> KVTLYKTTATADSDKFKISQILTFNFIKDKSYDKDTLVLKATGNINSGFVKPNPNDYDFSKLYWGAKYNVSISSQSNDSVNVVDYAPKNQNEEFQVQNTLGYTFGGNTAFSETINYKQESYRTTLSRNTNYKNVGWGVEAHKIMNNGWGPYGRDSFHPTYGNELFLAGRQSSAYAGQNFIAQHQMPLLSRSNFNPEFLSVLSHR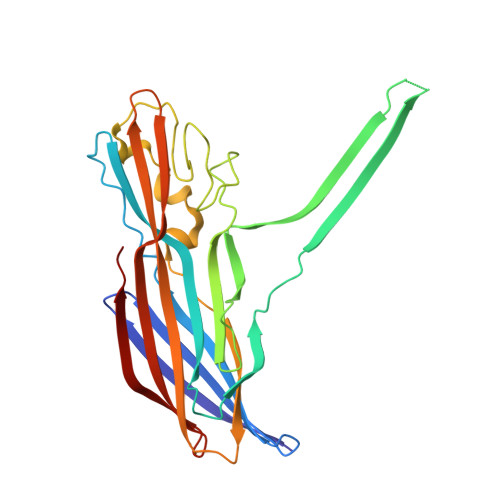QDGAKKSKITVTYQREMDLYQIRWNGFYWAGANYKNFKTRTFKSTYEIDWENHKVKLLDTKETENNK>MPGNNSAKGTATGNATALWRNAQLATLNPAMDGIGAVENAVIAVRNGRIAFAGPESDLPDDLSTADETTDCGGRWITPALIDCHTHLVFGGNRAMEFEMRLNGATYEEIAKAGGGIVSSVRDTRALSDEVLVAQALPRLDTLLSEGVSTIEIKSGYGLDIETELKMLRVARRLETLRPVRIVTSYLAAHATPADYKGRNADYITDVVLPGLEKAHAEGLADAVDGFCEGIAFSVKEIDRVFAAAQQRGLPVKLHAEQLSNLGGAELAASYNALSADHLEYLDETGAKALAKAGTVAVLLPGAFYA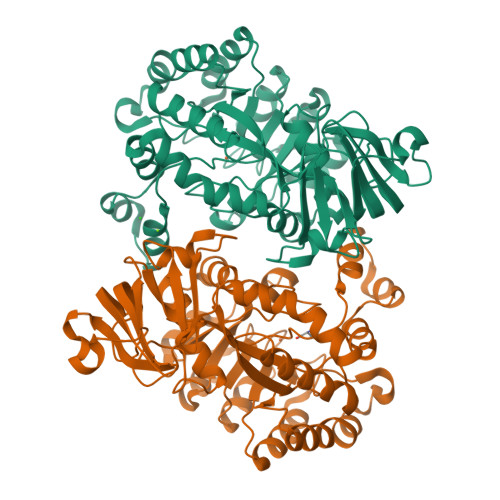LREKQLPPVQALRDAGAEIALATDCNPGTSPLTSLLLTMNMGATLFRMTVEECLTATTRNAAKALGLLAETGTLEAGKSADFAIWDIERPAELVYRIGFNPLHARIFKGQKVSP[2x]L and P function as the RNA polymerase complex, responsible for replicating and transcribing the viral genome. To catalyze the RNA synthesis in both replication and transcription, L sequentially consists of five domains: the RNA-dependent RNA polymerase domain (RdRp), polyribonucleotidyl transferase domain (PRNTase), connector domain (CD), methyltransferase domain (MTase), and C-terminal domain (CTD). P harbors an oligomerization domain (POD) for self-oligomerization, and the oligomeric P attaches to RdRp of L, tethering the polymerase to NC to extract the RNA strand for both replication and transcription. Here, we resolved two L–P complex conformations from the mumps virus (MuV), a typical member of nsNSVs, via cryogenic-electron microscopy.

One conformation presents all five domains of L, among which CD-MTase-CTD adopts a spatial organization distinct from PIV-5, with a continuous RNA tunnel from RdRp-PRNTase to CD-MTase-CTD, preferably as a transcription state. We then combined Lintegral–P particles from both unannealed and annealed particles and finally obtained a 3.02 Å cryo-EM structure. All five domains of L and regions of POD, PLinker2, and PCTD involved in L–P interfaces were clearly resolved. Different from the conserved RdRp-PRNTase, CD-MTase-CTD of MuV Lintegral–P adopts a spatial organization distinct from those of PIV-5, though their individual structures are pretty similar. The detailed alignment showed that MTase and CTD in MuV Lintegral–P appears as an integral on the PRNTase side instead of the RdRp side compared with PIV-5 L. The overall spatial organization of CD-MTase-CTD in MuV Lintegral–P is surprisingly similar to VSIV L. Actually, MuV Lintegral–P forms a continuous positively-charged tunnel from the GDN to the K-D-K-E motifs, ideal for the RNA synthesis followed by 5’ capping and methylation, which is favorable as the transcription state. Our Lintegral–P structure revealed four P molecules assembled into a helical bundle around RdRp of L via their respective POD. Different from the previous analysis on MuV P alone, four P molecules are more likely to adopt a parallel orientation in Lintegral–P. MuV Lintegral–P may bypass the MTase domain as one possible replication form. Models in (c, e) are the composite atomic models of MuV Lintegral–P and Lbody–P via rigid body docking of individual models into their respective composite cryo-EM maps, which are B-factor sharpened.

> MAGLNEILLPEVHLNSPIVRYKLFYYILHGQLPNDLEPDDLGPLANQNWKAIRAEESQVHARLKQIRVELIARIPSLRWTRSQREIAILIWPRILPILQAYDLRQSMQLPTVWEKLTQSTVNLISDGLERVVLHISNQLTGKPNLFTRSRAGQDTKDYSIPSTRELSQIWFNNEWSGSVKTWLMIKYRMRQLITNQKTGELTDLVTIVDTRSTLCIITPELVALYSSEHKALTYLTFEMVLMVTDMLEGRLNVSSLCTASHYLSPLKKRIEVLLTLVDDLALLMGDKVYGIVSSLESFVYAQLQYGDPVIDIKGTFYGFICNEILDLLTEDNIFTEEEANKVLLDLTSQFDNLSPDLTAELLCIMRLWGHPTLTASQAASKVRESMCAPKVLDFQTIMKTLAFFHAILINGYRRSHNGIWPPTTLHGNAPKSLIEMRHDNSELKYEYVLKNWKSISMLRIHKCFDASPDEDLSIFMKDKAISCPRQDWMGVFRRSLIKQRYRDANRPLPQPFNRRLLLNFLEDDRFDPIKELEYVTSGEYLRDPEFCASYSLKEKEIKATGRIFAKMTKRMRSCQVIAESLLANHAGKLMRENGVVLDQLKLTKSLLTMNQIGIISEHSRRSTADNMTLAHSGSNKHRINNSQFKKNKDNKHEMPDDGFEIAACFLTTDLTKYCLNWRYQVIIPFARTLNSMYGIPHLFEWIHLRLMRSTLYVGDPFNPPSDPTQLDLDTALNDDIFIVSPRGGIEGLCQKLWTMISISTIILSATEANTRVMSMVQGDNQAIAITTRVVRSLSHSEKKEQAYKASKLFFERLRANNHGIGHHLKEQETILSSDFFIYSKRVFYKGRILTQALKNVSKMCLTADILGDCSQASCSNLATTVMRLTENGVEKDLCYFLNAFMTIRQLCYDLVFPQTKSLSQDITNAYLNHPILISRLCLLPSQLGGLNFLSCSRLFNRNIGDPLVSAIADVKRLIKAGCLDIWVLYNILGRRPGKGKWSTLAADPYTLNIDYLVPSTTFLKKHAQYTLMERSVNPMLRGVFSENAAEEEEELAQYLLDREVVMPRVAHVILAQSSCGRRKQIQGYLDSTRTIIRYSLEVRPLSAKKLNTVIEYNLLYLSYNLEIIEKPNIVQPFLNAINVDTCSIDIARSLRKLSWATLLNGRPIEGLETPDPIELVHGCLIIGSDECEHCSSGDDKFTWFFLPKGIRLDDDPASNPPIRVPYIGSKTDERRVASMAYIKGASVSLKSALRLAGVYIWAFGDTEESWQDAYELASTRVNLTLEQLQSLTPLPTSANLVHRLDDGTTQLKFTPASSYAFSSFVHISNDCQILEIDDQVTDSNLIYQQVMITGLALIETWNNPPINFSVYETTLHLHTGSSCCIRPVESCVVNPPLLPVPLINVPQMNKFVYDPEPLSLLEMEKIEDIAYQTRIGGLDQIPLLEKIPLLAHLTAKQMVNSITGLDEATSIMNDAVVQADYTSNWISECCYTYIDSVFVYSGWALLLELSYQMYYLRIQGIQGILDYVYMTLRRIPGMAITGISSTISHPRILRRCINLDVIAPINSPHIASLDYTKLSIDAVMWGTKQVLTNISQGIDYEIVVPSESQLTLSDRVLNLVARKLSLLAIIWANYNYPPKVKGMSPEDKCQALTTHLLQTVEYVEYIQIEKTNIRRMIIEPKLTAYPSNLFYLSRKLLNAIRDSEEGQFLIASYYNSFGYLEPILMESKIFNLSSSESASLTEFDFILNLELSDASLEKYSLPSLLMTAENMDNPFPQPPLHHVLRPLGLSSTSWYKTISVLNYISHMKISDGAHLYLAEGSGASMSLIETFLPGETIWYNSLFNSGENPPQRNFAPLPTQFIESVPYRLIQAGIAAGNGIVQSFYPLWNGNSDITDLSTKTSVEYIIHKVGADTCALVHVDLEGVPGSMNSMLERAQVHALLITVTVLKPGGLLILKASWEPFNRFSFLLTVLWQFFSTIRILRSSYSDPNNHEVYIIATLAVDPTTSSFTTALNRARTLNEQGFSLIPPELVSEYWRKRVEQGQIIQDCIDKVISECVRDQYLADNNIILQAGGTPSTRKWLDLPDYSSFNELQSEMARLITIHLKEVIEILKGQASDHDTLLFTSYNVGPLGKINTILRLIVERILMYTVRNWCILPTQTRLTLRQSIELGEFRLRDVITPMEILKLSPNRKYLKSALNQSTFNHLMGETSDILLNRAYQKRIWKAIGCVIYCFGLLTPDVEGSERIDVDNDIPDYDIHGDII;>[4x]MDQFIKQDETGDLIETGMNVANHFLSTPIQGTNSLSKASILPGVAPVLIGNPEQKNIQHPTASHQGSKTKGRGSGVRSIIVSPSEAGNGGTQIPEPLFAQTGQGGIVTTVYQDPTIQPTGSYRSVELAKIGKERMINRFVEKPRTSTPVTEFKRGGPGAAAQGQTIQEEGIDGNGASAGSKERSGSLSGATLYAHLSLPQQDSTPANVGIAPQSAISANEIMDLLRGMDARLQHLEQKVDKVLAQGSMVTQIKNELSTVKTTLATIEGMMATVKIMDPGNPTGVPVDELRRSFSDHVTIVSGPGDVSFSSSEKPTLYLDELARPVSKPRPAKQTKSQPVKDLAGQKVMITKMITDCVANPQMKQAFEQRLAKASTEDALNDIKRDIIRSAI>[2x]SNAMFAPQGLAQFIKVNVTLENGEPVFIFTDANGQVCQGDITVTQAGTITYLLNDQTLKGLKFVGVGFVTPFDGIIDAVTISSDGMLVQLVDLDKTPG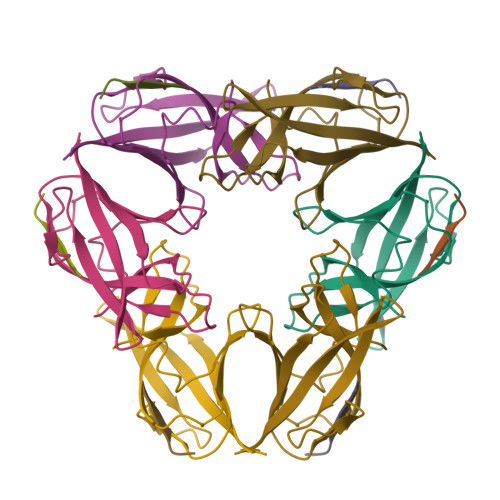TTKFQFVLSNTANTLLVLSPD;>[2x]PQIINRPQN GlxR from C. glutamicum (Cg-GlxR) has been identified as one of the central regulators of the Corynebacterium metabolism and more than 200 genes under GlxR control have so far been identified. Cg-GlxR, which shares a sequence identity of approximately 29% with CRP from E. coli (Ec-CRP), is a protein of 227 amino acids (compared to 210 for Ec-CRP) comprising an N-terminal dimerisation and ligand binding domain, and a C-terminal DNA-binding domain. The protein forms a homodimer with two structurally identical binding sites for cAMP. Once activated by cAMP, the regulator interacts with its target pseudo-palindromic DNA sites with the consensus sequence 5-TGTGANNTANNTCACA-3′ located in the regulatory region of Cg-GlxR controlled genes.

In order to shed further light on the activation mechanism and the structural and dynamic basis of allosteric regulation in the CRP/FNR family we determined the crystal structures of apo Cg-GlxR at a resolution of 2.5 Å. Apo Cg-GlxR crystallises in the monoclinic space group C2 with one homo-dimer in the asymmetric unit. Chain A shown on the left-hand side in blue is well defined with residues 1–226 (out of 227) present in the model, chain B (green) shows a larger degree of flexibility, and hence the model contains residues 3–164 and 178–217. The loop region of residues 165–177 that forms part of an anti-parallel β-sheet shows no density and was consequently not included. In addition, the model contains two phosphate ions with an occupancy of 0.5 in the cAMP binding site, two glycerol molecules at the protein surface and 72 water molecules. The two independent protein chains in the apo Cg-GlxR structure adopt a similar conformation with an rmsd of 1.36 Å for 200 equivalent Cα-atoms (all least-squares superpositions were calculated using the RAPIDO server). It is noteworthy that the DNA binding domains show a higher degree of flexibility as indicated by higher B-factors and a partial disorder of two external β-strands. All Cg-GlxR structures form symmetric homo-dimers. While apo Cg-GlxR is clearly more flexible compared to cAMP-bound form as indicated by partially disordered loops in one of the two independent DNA-binding domains the structural change caused by cAMP binding depicted in Figure 2 is smaller than observed for other members of the CRP/FNR family. Nevertheless, there is a significant movement changing the position of the DNA-binding helix in monomer A with respect to monomer B by up to 10 Å (measured by comparing equivalent Cα-positions of the DNA-binding helix in monomer B). This motion is more than enough to render the apo Cg-GlxR less suited for DNA-binding.

>MEGVQEILSRAGIFQGVDPTAVNNLIQDMETVRFPRGATIFDEGEPGDRLYIITSGKVKLARHAPDGRENLLTIMGPSDMFGELSIFDPGPRTSSAVCVTEVHAATMNSDMLRNWVADHPAIAEQLLRVLARRLRRTNASLADLIFTDVPGRVAKTLLQLANRFGTQEAGALRVNHDLTQEEIAQLVGASRETVNKALATFAHRGWIRLEGKSVLIVDTEHLARRAR[2x]>[2x]SAPS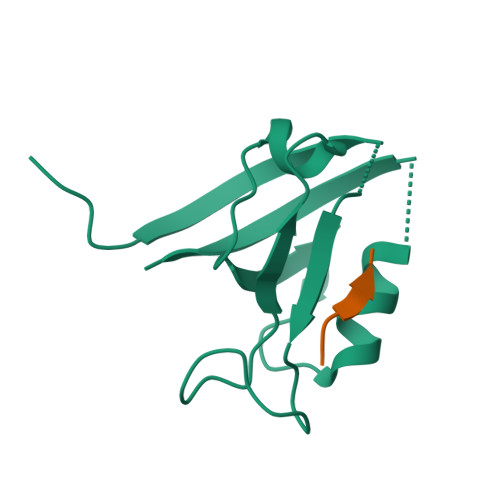VKGVSFDQANNLLIEPARIEEEELTLTILRQTGGLGISIAGGKGSTPYKGDDEGIFISRVSEEGPAARAGVRVGDKLLEVNGVALQGAEHHEAVEALRGAGTAVQMRVWRERM;>ARTIESEV[2x]>[2x]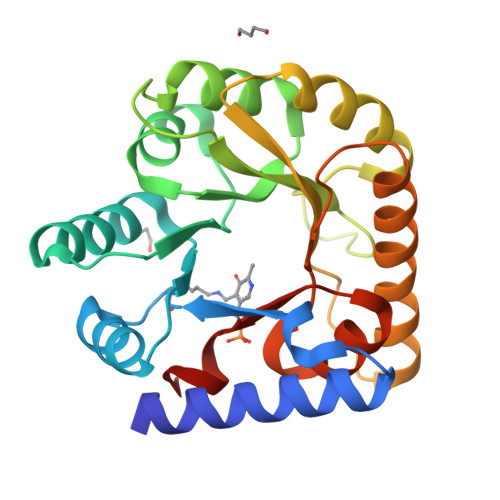MNDIAHNLAQVRDKISAAATRCGRSPEEITLLAVSKTAPASAIAEAIDAGQRQFGENYVQEGVDKIRHFQELGVTGLEWHFIGPLQSNKSRLVAEHFDWCHTIDRLRIATRLNDQRPAELPPLNVLIQINISDENSASGIQLAELDELAAAVAELPRLRLRGLMAIPAPESEYVRQFEVARQMAVAFAGLKTRYPHIDTLSLGMSDDMEAAIAAGSTMVRIGTAIFGARDYSAA>[24x]MSQLAHNLTLSIFDPVANYRAARIICT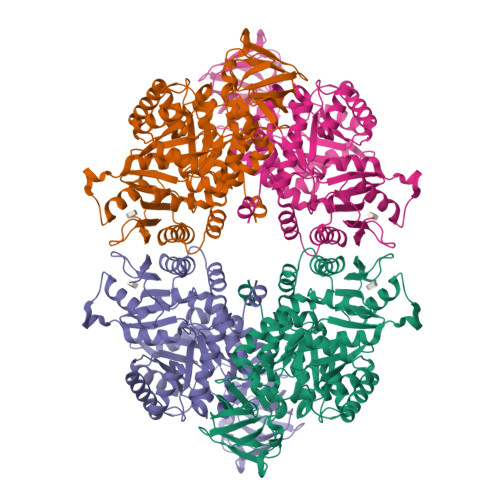IGPSTQSVEALKGLIQSGMSVARMNFSHGSHEYHQTTINNVRQAAAELGVNIAIALDTKGPEIRTGQFVGGDAVMERGATCYVTTDPAFADKGTKDKFYIDYQNLSKVVRPGNYIYIDDGILILQVQSHEDEQTLECTVTNSHTISDRRGVNLPGCDVDLPAVSAKDRVDLQFGVEQGVDMIFASFIRSAEQVGDVRKALGPKGRDIMIICKIENHQGVQNIDSIIEESDGIMVARGDLGVEIPAEKVVVAQKILISKCNVAGKPVICATQMLESMTYNPRPTRAEVSDVANAVFNGADCVMLSGETAKGKYPNEVVQYMARICLEAQSALNEYVFFNSIKKLQHIPMSADEAVCSSAVNSVYETKAKAMVVLSNTGRSARLVAKYRPNCPIVCVTTRLQTCRQLNITQGVESVFFDADKLGHDEGKEHRVAAGVEFAKSKGYVQTGDYCVVIHADHKVKGYANQTRILLVE>[16x]MTTVSCPANVITTTESDRIAGLFNIPAGIIPTGNVLSTIEVCAHRCIFDFFKQIRSDDNSLYSAQFDILLGTYCNTLNFVRFLELGLSVACICTKFPELAYVRDGVIQFEVQQPMIARDGPHPVDQPVHNYMVKRIHKRSLSAAFAIASEALSLLSNTYVDGTEIDSSLRIRAIQQMARNLRTVLDSFERGTADQLLGVLLEKAPPLSLLSPINKFQPEGHLNRVARAALLSDLKRRVCADMFFMTRHAREPRLISAYLSDMVSCTQPSVMVSRITHTNTRGRQVDGVLVTTATLKRQLLQ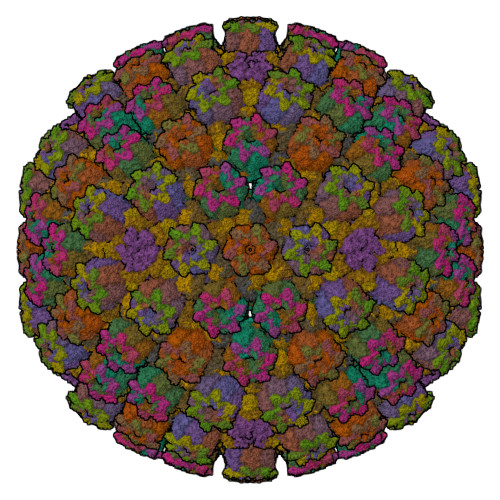GILQIDDTAADVPVTYGEMVLQGTNLVTALVMGKAVRGMDDVARHLLDITDPNTLNIPSIPPQSNSDSTTAGLPVNARVPADLVIVGDKLVFLEALERRVYQATRVAYPLIGNIDITFIMPMGVFQANSMDRYTRHAGDFSTVSEQDPRQFPPQGIFFYNKDGILTQLTLRDAMGTICHSSLLDVEATLVALRQQHLDRQCYFGVYVAEGTEDTLDVQMGRFMETWADMMPHHPHWVNEHLTILQFIAPSNPRLRFELNPAFDFFVAPGDVDLPGPQRPPEAMPTVNATLRIINGNIPVPLCPISFRDCRGTQLGLGRHTMTPATIKAVKDTFEDRAYPTIFYMLEAVIHGNERNFCALLRLLTQCIRGYWEQSHRVAFVNNFHMLMYITTYLGNGELPEVCINIYRDLLQHVRALRQTITDFTIQGEGHNGETSEALNNILTDDTFIAPILWDCDALIYRDEAARDRLPAIRVSGRNGYQALHFVDMAGHNFQRRDNVLIHGRPVRGDTGQGIPITPHHDREWGILSKIYYYIVIPAFSRGSCCTMGVRYDRLYPALQAVIVPEIPADEEAPTTPEDPRHPLHAHQLVPNSLNVYFHNAHLTVDGDALLTLQELMGDMAERTTAILVSSAPDAGAATATTRNMRIYDGALYHGLIMMAYQAYDETIATGTFFYPVPVNPLFACPEHLASLRGMTNARRVLAKMVPPIPPFLGANHHATIRQPVAYHVTHSKSDFNTLTYSLLGGYFKFTPISLTHQLRTGFHPGIAFTVVRQDRFATEQLLYAERASESYFVGQIQVHHHDAIGGVNFTLTQPRAHVDLGVGYTAVCATAALRCPLTDMGNTAQNLFFSRGGVPMLHDNVTESLRRITASGGRLNPTEPLPIFGGLRPATSAGIARGQASVCEFVAMPVSTDLQYFRTACNPRGRASGMLYMGDRDADIEAIMFDHTQSDVAYTDRATLNPWASQKHSYGDRLYNGTYNLTGASPIYSPCFKFFTPAEVNTNCNTLDRLLMEAKAVASQSSTDTEYQFKRPPGSTEMTQDPCGLFQEAYPPLCSSDAAMLRTAHAGETGADEVHLAQYLIRDASPLRGCLPLPR;>[15x]MTQPASSRVVFDPSNPTTFSVEAIAAYTPVALIRLLNASGPLQPGHRVDIADARSIYTVGAAASAARARANHNANTIRRTAMFAETDPMTWLRPTVGLKRTFNPRIIRPQPPNPSMSLGISGPTILPQKTQSADQSALQQPAALAFSGSSPQHPPPQTTSASVGQQQHVVSGSSGQQPQQGAQSSTVQPTTGSPPAAQGVPQSTPPPTQNTPQGGKGQTLSHTGQSGNASRSRRV;>MGSQPTNSHFTLNEQTLCGTNISLLGNNRFIQIGNGLHMTYAPGFFGNWSRDLTIGPRFGGLNKQPIHVPPKRTETASIQVTPRSIVINRMNNIQINPTSIGNPQVTIRLPLNNFKSTTQLIQQVSLTDFFRPDIEHAGSIVLILRHPSDMIGEANTLTQAGRDPDVLLEGLRNLFNACTAPWTVGEGGGLRAYVTSLSFIAACRAEEYTDKQAADANRTAIVSAYGCSRMETRLIRFSECLRAMVQCHVFPHRFISFFGSLLEYTIQDNLCNITAVAKGPQEAARTDKTSTRRVTANIPACVFWDVDKDLHLSADGLKHVFLVFVYTQRRQREGVRLHLALSQLNEQCFGRGIGFLLGRIRAENAAWGTEGVANTHQPYNTRALPLVQLSNDPTSPRCSIGEITGVNWNLARQRLYQWTGDFRGLPTQLSCMYAAYTLIGTIPSESVRYTRRMERFGGYNVPTIWLEGVVWGGTNTWNECYY[5x];>[10x]MAMPFEIEVLLPGELSPAETSALQKCEGKIITFSTLRHRASLVDIALSSYYINGAPPDTLSLLEAYRMRFAAVITRVIPGKLLAHAIGVGTPTPGLFIQNTSPVDLCNGDYICLLPPVFGSADSIRLDSVGLEIVFPLTIPQTLMREIIAKVVARAVERTAAGAQILPHEVLRGADVICYNGRRYELETNLQHRDGSDAAIRTLVLNLMFSINEGCLLLLALIPTLLVQGAHDGYVNLLIQTANCVRETGQLINIPPMPRIQDGHRRFPIYETISSWISTSSRLGDTLGTRAILRVCVFDGPSTVHPGDRTAVIQV>SMACYGGFDLYFILDKSGSVLHHWNEIYYFVEQLAHKFISPQLRMSFIVFSTRGTTLMKLTEDREQIRQGLEELQKVLPG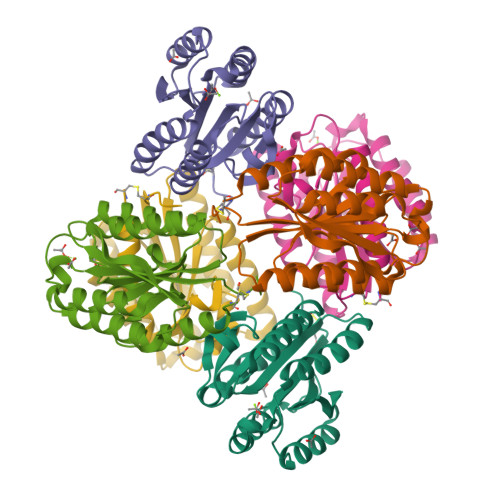GDTYMHEGFERASEQIYYENRQGYRTASVIIALTDGELHEDLFFYSEREANRSRDLGAIVYAVGVKDFNETQLARIADSKDHVFPVNDGFQALQGIIHSILKKSC[6x]>[2x]MGSSHHHHHHSQGSMHYLDNLLLNTDSYKASHWLQYPPGTDASFFY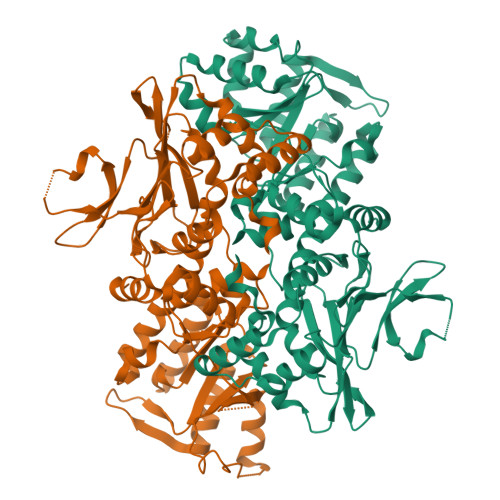VESRGGVYDQTAFFGLQSILKEAINRPVTHADIDDAKALLAAHGEPFNEAGWRDIVDRLGGQLPIRIRAVPEGCVVPTHNVLMTIESTDAKAFWVPSYLETLLLRVWYPVTVATVSWQVKQIVRDFLQRTSDDPEGQLPFKLFDFGARGVSSLGSAALGGAAHLVNFLGTDTLSALLLARAHYHTPVAGYSFPAAEHSTITSWGREREVDAYRNMLTQFARPGAIVAVVSDSYDIYRAIREHWGTTLREEIIASGATVFIRPDSGDPVDVVEQCLLLLDEAFGHQVNGKGYKVLNHVRVFQGDGINPQSLRAILERITAAGYAADNVAFGMGGALLQKVDRDTQKFALKCSAVRVDGAWIDVYKDPITDQGKQSKRGRLTLLRDRATGQYRSALLDEVATHAGDSDDALVTVWENGQMLREWTLEQVRAHADAARL> GSNRRL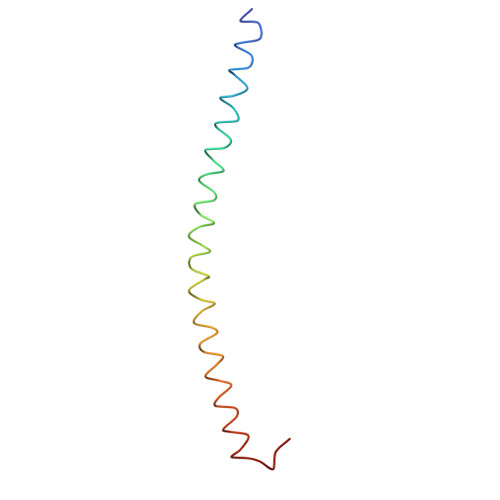QQTQAQVDEVVDIMRVNVDKVLERDQKLSELDDRADALQAGASQFETSAAKLKRKYWWKN> GAMGKLCENQQEIYAAYRVANLLGVYEDCSPNGFYQRWKQKNAFMKAQAEEFGIGSTDHFIDDVERIVDQRRAETEWKNADAWKNGTAAFGARYLTPEMYLDYELKSIQLAFATYKGELVGNHKCHVYTEDEKRAFYDANQDLFTRYHGDLFSYEEVDLIIEKWLKVQEYQDIIESVVANTHLNETTVNEISAQDVSDEKSDNAVRWITEFEKIWNQMQEEKRLREDKSCPEETKSESSIGNCGHCYYVSSIHGDDANDGTEDQPLKSLYAVNRLDLQPGDQVLLERGSVFENQFLHLNVQGTKEQPIYIGAYGNGAKPLIQTNGQGIWYQDYGNELDAPTHVYRGYVSSAVLLYDCEYLTVENLEISNKGGVFGETYSAPHKMNRTGVAGIAKNRGTLHEIHLSNLYIHDVEGNVYDKHMNNGGIYFT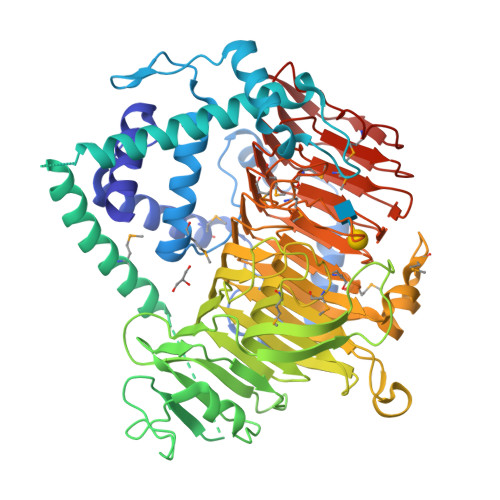CLKPEAEEKTGVARYENVSVRGCHLKRTSRWGIAVGYSYKCKEFMTAELPDELFERYGHHNIYIADNYVEEIGGDGITVMYAMKPLVEYNSGDSCALEMNDRYYTEPEDRAGKVAAGIWPWKCKDALLTYNEMRDMRLNQDSMAWDADSGDGTLYQYNYSHLNEGGCVMFCLEEAIHNEFRYNVSVDDLGGLISPSGNPDAWIHHNVFYRRAEVPFVRPHMDDGKYVAEENEIHLI>TTVTIVRKDGRIAIAADTLTKWGGGKESADYVANHEKIIRVGDSYVAITGSATFKLILADYFASLDEPPQLDSVARIFCVWNTLHGALKEHYYLQAGEDKEDDLESSRMDVLIANPRGIFGVAAHRTVQEFSKFYAYGSGSPYALGAMYAAYRAPSLDAEAVARLGVMAAAEFHDESGLPVQSFVMELSPDVGSGENLYFQ[7x]

The second hitherto unknown bacterial proteasome family member was primarily found in Betaproteobacteria, hence its name BPH, short for Betaproteobacterial proteasome homologue. In this study, we present the first experimental characterization of two bacterial BPH proteins. Their crystal structures reveal homo-oligomeric double-barrel complexes with internalized active sites akin to those of proteasome and HslV. Unique structural features, however, like an elongated inner pore loop with a highly acidic sequence, distinguish BPH from its relatives. Confirming an initial hypothesis, our cluster analysis shows that BPH branches off from HslV and appears to be its direct descendant.

To ascertain the functional nature of the BPH active site, we covalently modified it with the proteasome-specific inhibitor epoxomicin. This compound features an epoxyketone electrophilic trap, the warhead, which renders it highly selective toward the catalytic Thr-1 of proteasome-like proteins. Additionally, we obtained co-crystals of Td-BPH with bound epoxomicin diffracting to 2.95 Å, whose structure could be solved on the basis of the apo Td-BPH coordinates. Epoxomicin is bound in all subunits, in the same fashion as in comparable co-structures with epoxomicin, which are only available for the proteasome but not for HslV or Anbu. The peptide-like moiety lines up in the substrate binding pocket to form an additional β-strand to the S3–S4 β hairpin, as in the proteasome. In particular, the modification of Td-BPH Thr-1 by the epoxomicin warhead confirms this residue as the active nucleophile in the catalytic reaction cycle. Further, an interesting peculiarity of the inhibitor-bound structure concerns the pore loop. Although the central portion of this loop is unresolved in the ligand-free Td-BPH structure, a mostly continuous electron density is observed for the whole loop in the bound structure, allowing to approximately trace its backbone. The center portion of the loop is closed over the epoxomicin peptide-like moiety. It is therefore conceivable that the loop contributes to substrate recognition, adopting a well-defined conformation and forming specific interactions with yet to be identified native substrates.Here, we study DHPS-3-dehydrogenase from Cupriavidus pinatubonensis (CpHpsN), a bacterium capable of utilizing DHPS as a sole carbon source. Kinetic analysis of CpHpsN reveals a strict preference for R-DHPS, catalyzing its 4-electron oxidation to R-SL, with high specificity for NAD+ over NADP+. CpHpsN forms a domain-swapped tight dimer with 28% of surface area buried at the dimer interface, with the interface featuring extensive hydrophobic and hydrogen-bond interactions. Domain 4 lies at the C-terminus and contributes to the active site and is also involved in dimerization through a metal binding site. Coordination of Zn2+ involves three residues from one monomer and one residue (His411*; * denotes the other monomer in the dimer) from the other monomer (Fig. 5 and S7†), showing that the enzyme forms an obligate dimer.

To probe the roles of Glu318, His319 and Asp352, we conducted site-directed mutagenesis to convert each residue independently to Ala. The E318A and H319A mutants of CpHpsN suffered 580-fold and 240-fold reductions in (kcat/KM)app values, respectively, which was mainly due to a reduction in kappcat values (Fig. S11† and Table 2). The 3D structure of the ‘closed’ CpHpsN H319A·Zn2+·NADH·R-DHPS complex displays a productive geometry with the primary hydroxyl carbon of DHPS positioned 3.3 Å away from C4 of the nicotinamide group. In this complex, the Zn and R-DHPS sites are not fully occupied, and the final coordinates are modelled with the occupancy of 0.7, whereas the cofactor NADH has a full occupancy. The partial occupancy of zinc presumably arises due to incomplete reconstitution during purification. However, the concentration of R-DHPS used during crystallization was in excess (>100×) and is not a limiting factor. This observation therefore suggests that zinc is essential for ligand binding in the active site.

>[2x]GMISYLKKAEKTPQTETATAQKVVTEMLAEIQARGKDAVRQYAKQLDGWSGDIVLTPDQIREQTKDVPAGVRADIDFAIRQVTDFALAQRESLKEFSVELHPGVTAGQRVLPVNVVGCYAPAGRYAHIASAYMGVATAKAAGVKTVVACSSPFRGQGIHPHVLYAFQAAGADVIMALGGVQAIASMAYGLFTGKPADVVVGPGNKFVAEAKRSLYGQVGIDVFAGPSEVAVIADETADPAIVASDLVGQAEHGHESPAWLFTTSRDLADRVMALVPELIAKLPPTARDAATAAWRDYGEVILCGTREEVVEISDRYASEALEVHTADLDWWLANLTCYGSLFLGEETTVAFGDKTSGPNHVLPTKGAARYSGGLSVHKFMKTLTWQQMTREATRQIGQVTARISRLEGMEAHARTADDRMAKYFPNASFEMGTPVEV>MSKPQPIAAANWKCNGSQQSLSELIDLFNSTSINHDVQCVVASTFVHLAM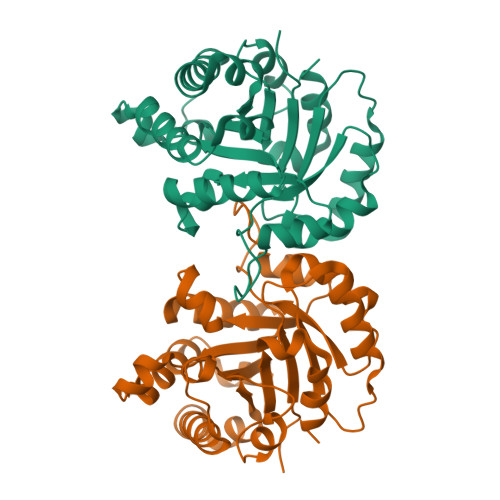TKERLSHPKFVIAAQNAIAKSGAFTGEVSLPILKDFGVNWIVLGHSERRAYYGETNEIVADKVAAAVASGFMVIACIGETLQERESGRTAVVVLTQIAAIAKKLKKADWAKVVIAYEAVWAIGTGKVATPQQAQEAHALIRSWVSSKIGADVAGELRILYGGSVNGKNARTLYQQRDVNGFLVGGASLKPEFVDIIKATQ[2x]(1R,3r,5S)-bicyclo[3.1.0]hexan-3-yl [(2R,6S,12Z,13aS,14aR,16aS)-2-{[6-methoxy-3-(trifluoromethyl)quinoxalin-2-yl]oxy}-14a-{[(1-methylcyclopropyl)sulfonyl]carbamoyl}-5,16-dioxo-1,2,3,5,6,7,8,9,10,11,13a,14,14a,15,16,16a-hexadecahydrocyclopropa[e]pyrrolo[1,2-a][1,4]diazacyclopentadecin-6-yl]carbamate | C39 H47 F3 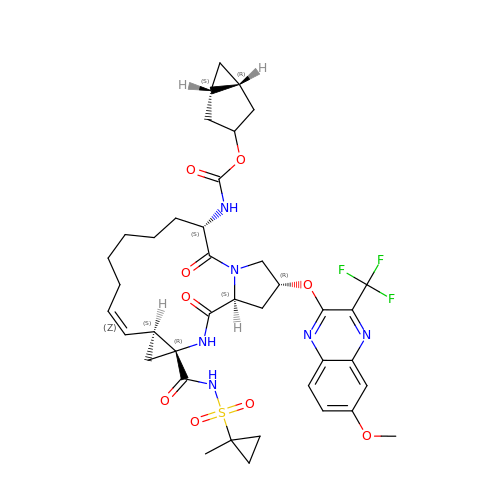N6 O9 S | CEAGGSVWMLUKOY-HDLCAPKFSA-N>QDADKLPHTKVTLVAPPQVHPHEQATKSGPKVVEFTMTIEEKKMVIDDKGTTLQAMTFNGSMPGPTLVVHEGDYVQLTLVNPATNAMPHNVDFHGATGAL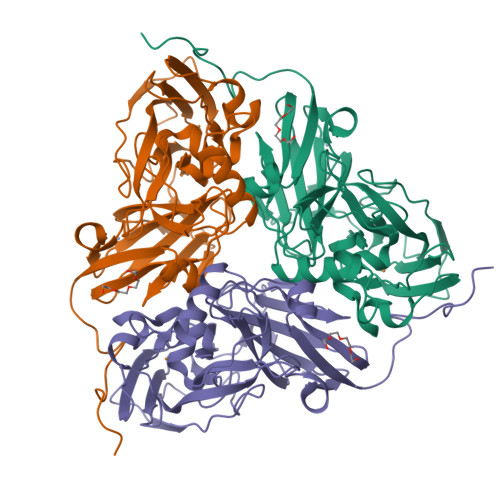GGAKLTNVNPGEQATLRFKADRSGTFVYHCAPEGMVPWHVVSGMSGTLMVLPRDGLKDPQGKPLHYDRAYTIGEFDLYIPKGPDGKYKDYATLAESYGDTVQVMRTLTPSHIVFNGKVGALTGANALTAKVGETVLLIHSQANRDTRPHLIGGHGDWVWETGKFANPPQRDLETWFIRGGSAGAALYTFKQPGVYAYLNHNLIEAFELGAAGHIKVEGKWNDDLMKQIKAPAPIPR[2x]> MPAIMTMLADHAARQLLDFSQKLDINLLDNVVNCLYHGEGAQQRMAQEVLTHLKEHPDAWTRVDTILEFSQNMNTKYYGLQILENVIKTRWKILPRNQCEGIKKYVVGLIIKTSSDPTCVEKEKVYIGKLNMILVQILKQEWPK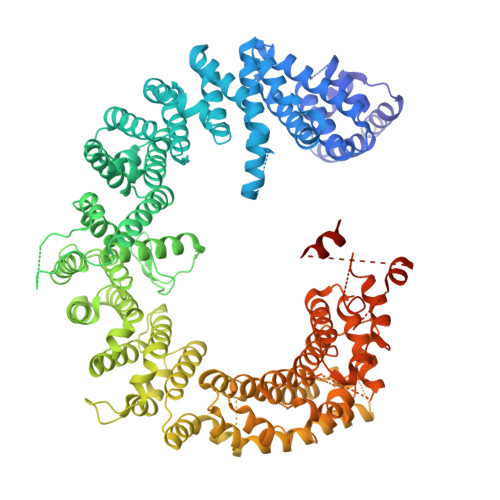HWPTFISDIVGASRTSESLCQNNMVILKLLSEEVFDFSSGQITQVKSKHLKDSMCNEFSQIFQLCQFVMENSQNAPLVHATLETLLRFLNWIPLGYIFETKLISTLIYKFLNVPMFRNVSLKCLTEIAGVSVSQYEEQFVTLFTLTMMQLKQMLPLNTNIRLAYSNGKDDEQNFIQNLSLFLCTFLKEHDQLIEKRLNLRETLMEALHYMLLVSEVEETEIFKICLEYWNHLAAELYRESPFSTSASPLLSGSQHFDVPPRRQLYLPMLFKVRLLMVSRMAKPEEVLVVENDQGEVVREFMKDTDSINLYKNMRETLVYLTHLDYVDTERIMTEKLHNQVNGTEWSWKNLNTLCWAIGSISGAMHEEDEKRFLVTVIKDLLGLCEQKRGKDNKAIIASNIMYIVGQYPRFLRAHWKFLKTVVNKLFEFMHETHDGVQDMACDTFIKIAQKCRRHFVQVQVGEVMPFIDEILNNINTIICDLQPQQVHTFYEAVGYMIGAQTDQTVQEHLIEKYMLLPNQVWDSIIQQATKNVDILKDPETVKQLGSILKTNVRACKAVGHPFVIQLGRIYLDMLNVYKCLSENISAAIQANGEMVTKQPLIRSMRTVKRETLKLISGWVSRSNDPQMVAENFVPPLLDAVLIDYQRNVPAAREPEVLSTMAIIVNKLGGHITAEIPQIFDAVFECTLNMINKDFEEYPEHRTNFFLLLQAVNSHCFPAFLAIPPTQFKLVLDSIIWAFKHTMRNVADTGLQILFTLLQNVAQEEAAAQSFYQTYFCDILQHIFSVVTDTSHTAGLTMHASILAYMFNLVEEGKISTSLNPGNPVNNQIFLQEYVANLLKSAFPHLQDAQVKLFVTGLFSLNQDIPAFKEHLRDFLVQIKEFAGEDTSD> KHLPEPFRIRVIEPVKRTTRAYREEAIIKSGMNPFLLDSEDVFIDLLTDSGTGAVTQSMQAAMMRGDEAFSGSRSYYALAESVKNIFGYQYTIPTHQGRGAEQIYIPVLIKKREQEKGLDRSKMVAFSNYFFDTTQGHSQINGCTVRNVYIKEAFDTGVRYDFKGNFDLEGLERGIEEVGPNNVPYIVATITSNSAGGQPVSLANLKAMYSIAKKYDIPVVMDSARFAE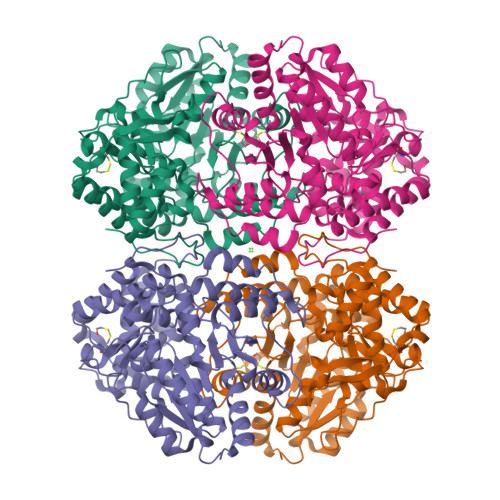NAYFIKQREAEYKDWTIEQITRETYKYADMLAMSAKKDAMVPMGGLLCMKDDSFFDVYTECRTLCVVQEGFPTYGGLEGGAMERLAVGLYDGMNLDWLAYRIAQVQYLVDGLEEIGVVCQQAGGHAAFVDAGKLLPHIPADQFPAQALACELYKVAGIRAVEIGSFLLGRDPKTGKQLPCPAELLRLTIPRATYTQTHMDFIIEAFKHVKENAANIKGLTFTYEPKVLRHFTAKLKEV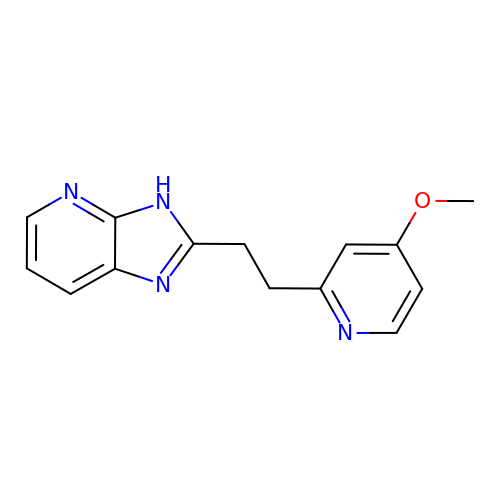2-[2-(4-methoxypyridin-2-yl)ethyl]-3H-imidazo[4,5-b]pyridine | C14 H14 N4 O | YBOCDKFRGBOOFO-UHFFFAOYSA-N> GSHMIEVVCNDRLGKKVRVKCNTDDTIGDLKKLIAAQTGTRWNKIVLKKWYTIFKDHVSLGDYEIHDGMNLELY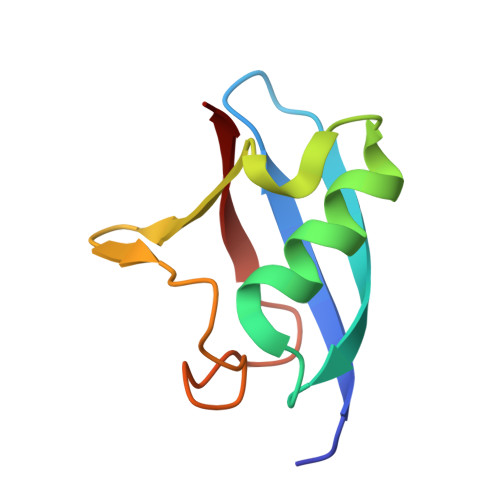YQ> MDFSKLPKIRDEDKESTFGYVHGVSGPVVTACDMAGAAMYELVRVGHSELVGEIIRLEGDMATIQVYEETSGVSVGDPVLRTGKPLSVELGPGIMGAIFDGIQRPLSDISSQTQSIYIPRGVNVSALSRDVKWDFTPCKNLRVGSHITGGDIYGIVNENSLIKHKIMLPPRNRGTVTYIAPPGNYDTSDVVLELEFEGIKEKFSMVQVWPVRQVRPVTEKLPANHPLLTGQRVLDALFPCVQGGTTAIPGAFGCGKTVISQSLSKYSNSDVIIYVGCGERGNEMSEVLRDFPELTMEVDGKVESIMKRTALVANTSNMPVAAREASIYTGITLSEYFRDMGYHVSMMADSTSRWAEALREISGRLAEMPADSGYPAYLGARLASFYERAGRVKCLGNPEREGSVSIVGAVSPPGGDFSDPVTSATLGIVQVFWGLDKKLAQRKHFPSVNWLISYSKYMRA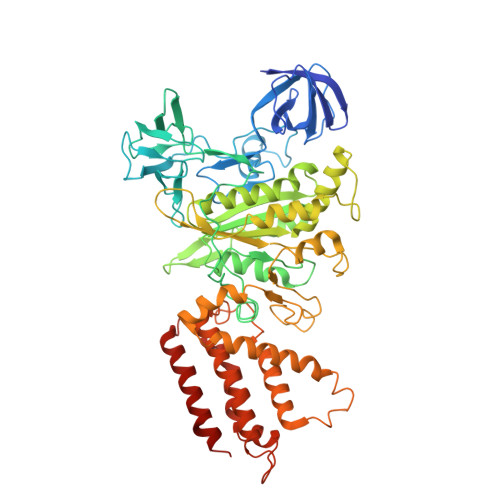LDEYYDKHFTEFVPLRTKAKEILQEEEDLAEIVQLVGKASLAETDKITLEVAKLIKDDFLQQNGYTPYDRFCPFYKTVGMLSNMIAFYDMARRAVETTAQSDNKITWSIIREHMGEILYKLSSMKFKDPVKDGEAKIKADYAQLLEDMQNAFRSLED> SNAMATLVSNWSTNNVSESFIAPLEKRAEKDVALGNDVPIIDLQQDHLLIVQQITKACQDFGLFQVINHGVPEKLMVEAMEVYKEFFALPAEEKEKFQPKGEPAKFELPLEQKAKLYVEGERRCNEEFLYWKDTLAHGCYPLHEELLNSWPEKPPTYRDVIAKYSVEVRKLTMRILDYICEGLGLKLGYFDNELTQIQMLLANYYPSCPDPSTTIGSGGHYDGNLITLLQQDLVGLQQLIVKDDKWIAVEPIPTAFVVNLGLTLKVMSNEKFEGSIHRVV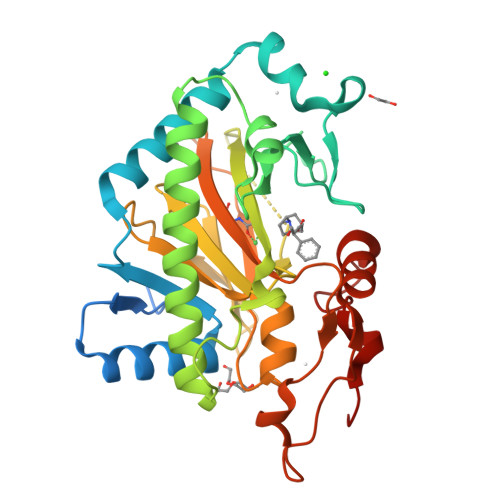THPIRNRISIGTLIGPDYSCTIEPIKELISQENPPLYKPYPYAEFAEIYLSDKSDYDAGVKPYKINQFPN> GPQDNPYERGPDPTEDSIEAIRGPFSVATERVSSFASGFGGGTIYYPRETDEGT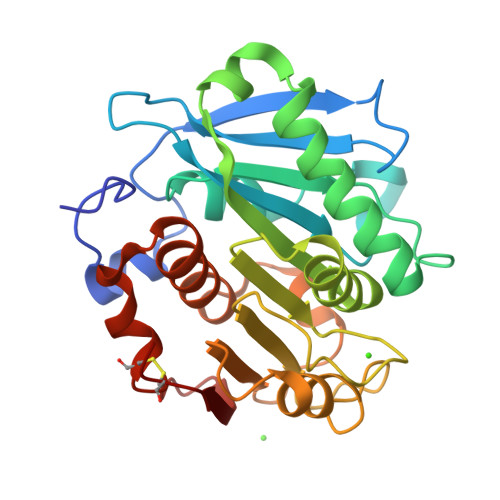FGAVAVAPGFTASQGSMSWYGERVASQGFIVFTIDTNTRLDQPGQRGRQLLAALDYLVERSDRKVRERLDPNRLAVMGHAMGGGGSLEATVMRPSLKASIPLTPWNLDKTWGQVQVPTFIIGAELDTIAPVSTHAKPFYESLPSSLPKAYMELDGATHFAPNIPNTTIAKYVISWLKRFVDEDTRYSQFLCPNPTDRAIEEYRSTCPY> CW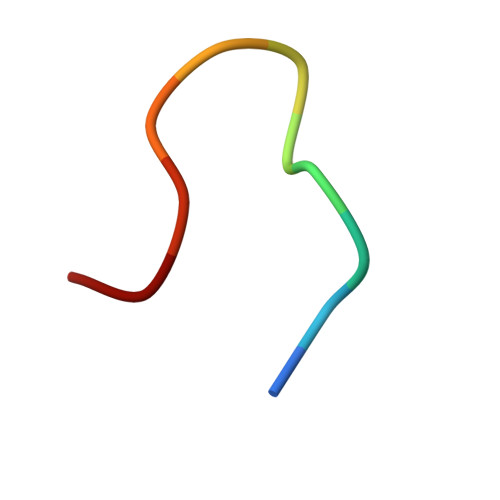WKKKKKWWC>GVKTFQFPFAEQLEKVAEQFPTFQILNEEGEVVNEEAMPELSDEQLKELMRRMVYTRILDQRSISLNRQGRLGFYAPTAGQEASQIASHFALEKEDFILPGYRDVPQIIWHGLPLYQAFLFSRGHFHGNQIPEGVNVLPPQIIIGAQYIQAAGVALGLKMRGKKAVAITYTGDGGTSQGDFYEGINFAGAFKAPAIFVVQNNRFAISTPVEKQTVAKTLAQKAVAAGIPGIQVDGMDPLAVYAAVKAARERAINGEGPTLIETLCFRYGPHTMSGDDPTRYRSKELENEWAKKDPLVRFRKFLEAKGLWSEEEENNVIEQAKEEIKEAIKKADETPKQKVTDLISIMFEELPFNLKEQYEIYKEKESK[4x];>[4x]AQMTMVQAITDALRIELKNDPNVLIFGEDVGVNGGVFRATEGLQAEFGEDRVFDTPLAESGIGGLAIGLALQGFRPVPEIQFFGFVYEVMDSICGQMARIRYRTGGRYHMPITIRSPFGGGVHTPELHSDSLEGLVAQQPGLKVVIPSTPYDAKGLLISAIRDNDPVIFLEHLKLYRSFRQEVPEGEYTIPIGKADIKREGKDITIIAYGAMVHESLKAAAELEKEGISAEVVDLRTVQPLDIETIIGSVEKTGRAIVVQEAQRQAGIAANVVAEINERAILSLEAPVLRVA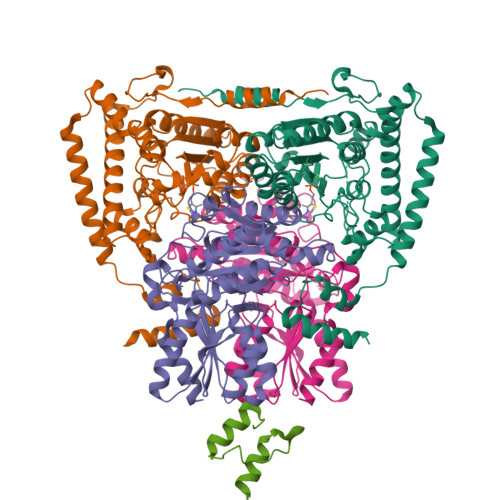APDTVYPFAQAESVWLPNFKDVIETAKKVMNF;>[2x]AGPNRRVIAMPSVRKYAREKGVDIRLVQGTGKNGRVLKEDIDAFLAGGA>[2x]MRFQYQALLNEHQSQLDRFSSHIVATLDKYAHIPHLISKDKELVDALLSAQNSAQIDITNRYLEQVNEVIQA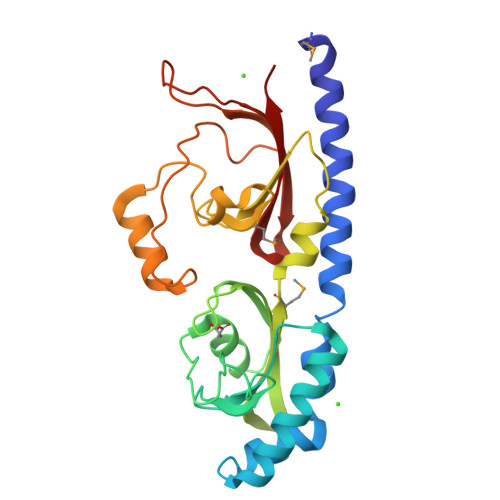ADTYLIDRFGNTIASSNWNLDRSFIGRNFAWRPYFYLSIAGQKSQYFALGSTSGQRGYYYAYPVIYAAEILGVIVVKMDLSAIEQGWQNKSSYFVATDDHQVVFMSSQPAWLFHSVADLSPAQLNDIRQSQQYLDSPIPSLGWQGDLQAEQSEWRKPEKHWLQDDYIVSSRPLPELALTIRVLSPKIE In bacteria, Ser/Thr protein kinase-like sequences are found as part of large multidomain polypeptides that biosynthesize lanthipeptides, a class of natural products distinguished by the presence of thioether cross-links. The kinase domain phosphorylates Ser or Thr residues in the peptide substrates. Subsequent β-elimination by a lyase domain yields electrophilic dehydroamino acids, which can undergo cyclase domain-catalyzed cyclization to yield conformationally restricted, bioactive compounds. We also describe the first crystal structures of a class III lanthipeptide synthetase, consisting of the lyase, kinase, and cyclase domains, in various states including complexes with its leader peptide and nucleotide.

Reasoning that heterogeneity in the stoichiometry of ThurKC with bound precursor peptide may contribute to the poor crystal quality, we generate a single-chain fusion of the ThurA1 leader peptide attached to the N-terminus of ThurKC with poly(-Gly-Ser-) linkers of various lengths. The most suitable fusions consisted of either seven or ten residues separating the leader peptide and ThurKC, hereafter termed LP-(GS)X-ThurKC, where X represents the number of residues in the linker. Nonetheless, these experiments show fusion of the leader sequence to the ThurKC lanthipeptide synthetase yielded a constitutively active enzyme that could act on peptide substrates without a leader in vitro and in vivo, as has been demonstrated for a leader peptide-catalytic domain fusion of class II LctM34 and the unrelated YcaO heterocyclases involved in cyanobactin biosynthesis. The single-chain LP-(GS)7-ThurKC fusion yielded easily reproducible crystals that reproducibly diffracted to resolutions beyond 2.5 Å. A preliminary model consisting of ∼70% of the scattering atoms was used to phase and build using a 2.15 Å resolution native data set collected on crystals of LP-(GS)7-ThurKC bound to ATP and Ca2+ (as a surrogate for Mg2+). There are two copies in the crystallographic asymmetric unit and continuous density can be observed for both polypeptides throughout their entire lengths except for segments Asp(−10) of leader peptide to Glu2 of ThurKC, residues Arg24–Asn28, and Ser214–Glu222, which are all presumably disordered. The overall structure of LP-(GS)7-ThurKC resembles a cupped hand with the lyase and kinase domains forming the fingers and the cyclase domain forming the palm and thumb. First, clear and continuous electron density can be observed for the leader peptide corresponding to residues Met(−22) to Asp(−10), and this accounts for all but the C-terminal ten residues of the leader peptide. Lastly, residues Asn4 through Ile21 form a short α-helix (hereafter, the N-helix) followed by a turn and interact with all three domains, suggesting that it allows for functional interplay between the domains.

>[2x]SNAMNTVLELQKLAHDTEGKGQAAESGSGSGSMEGNMLYHRYLKPNSEYYKKIEVRGKDNIYELNDIPDTYAVFLDNESVWKHYHVKGSTLPEQGWKIHVTSSLEDSKDVLDKVARLCIDKKIEFKHLKDKDSFMKMNSKNANRASSGKFITIYPTNNEVFVELLEMISLAIQDFKKGPYILNDKRWKNSNVFYRYGGFKGIFNEHGEHCIRDKEGNLIKDQRNPFYQVPDFVKDFDDYLNTINNSGELENKGESRLGKYKIETALSFSNAGGVYLATRKKDNLKVIIKEARPSAGLDGAAQDALARQKIEYDALKKLKDVSGVVNLIEYFQEWEHYFLVEEFIEGRDLRQWIAQEFPFFEDNNGMSNHIKDVKMILLQLLDLIDSMHNQGVAMGDLQPANIMVTEDLTVRIIDFETAMPVNSDDRPAMLTTGFVSHEMKVSGARDWFGFKRLVRYLALPVLTSEDLEGYLQYNHLNWIKENYGYEFYSFIVDLQEKCDKRIKDYQTFIPKEINLNDQTSDFNLTSIINKLIIGVESSLTNDERFINGDIRQFEMNGGKFNFLTGGSGAAFTLTKNKSSIAEVDKWIQSVLLDNLPLIEEDGLFTGKTGILALLYDKGYKEVVLNELKILKDNINQTDISIRSGLSGIGLFVISLYLETENKEYLKLAKDLERMIKLNRAKDKQLKVKDWMAVDIGVIDGLSGVSLFYSALYSVTQNQKYLEEAEVLIKEDLESTKKDDVTGVLQTVDNKNRLLPYLSGGSIGVAISIWFLNHVSGQDLYREEMNSILKLSKTRCTISGGLFDGAGSFLLIPSMVKNDKNREVILNEVLNLLNIFLIEKNSYYVYPGQFSYRLADDVYTGSSGIILALMGVIKGNPLYWLPLVNSDEFLARTKVKDLSVTSGKI> DTFSERTLGLNSIDNTEI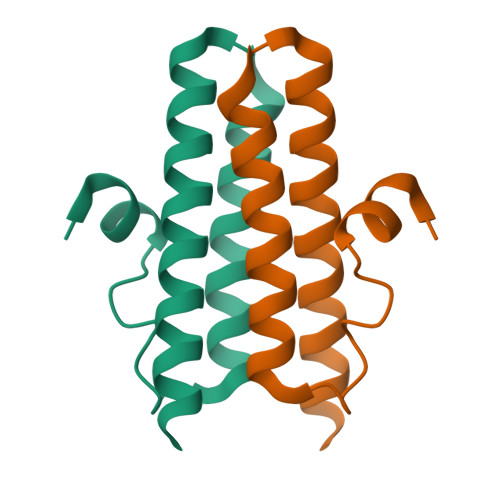SEVVSLGLVSSALDKITGLLSADNLSETVSQARDFSHTLSKSLKSRAKSLSQK>[4x]FQSMNRSALDFRHFVDHLRRQGDLVDVHTEVDANLEIGAITRRVYERRAPAPLFHNIRDSLPGARVLGAPAGLRADRARAHSRLALHFGLPEHSGPRDIVAMLRAAMRAEPIAPRRLERGPVQENVWLGEQVDLTRFPVPLLHEQDGGRYFGTYGFHVVQTPDGSWDSWSVGRLMLVDRNTLAGPTIPTQHIGIIREQWRRLGKPTPWAMALGAPPAALAAAGMPLPEGVSEAGYVGALVGEPVEVVRTQTNGLWVPANTEIVLEGEISLDETALEGPMGEYHGYSFPIGKPQPLFHVHALSFRDQPILPICVAGTPPEEHHTIWGTMISAQLLDVAQNAGLPVDMVWCSYEAATCWAVLSIDVQRLAALGTDAAAFAARVAETVFGSHAGHLVPKLILVGNDIDVTEIDQVVWALATRAHPLHDHFAFPQIRDFPMVPYLDAEDKARGSGGRLVINCLYPEQFAGQMRAATASFRHAYPTALRRRVEERWSDYGFGDA

The UbiD family of reversible (de)carboxylases depends on the recently discovered prenylated-FMN (prFMN) cofactor for activity. Here, we show that the Pseudomonas aeruginosa virulence attenuation factor PA0254/HudA is a pyrrole-2-carboxylic acid decarboxylase. We here report that the UbiD-like Pseudomonas aeruginosa virulence attenuation factor PA0254/HudA is a close homologue of Bacillus megaterium PYR2910 pyrrole-2-carboxylate (P2C) decarboxylase and show that PA0254 is capable of prFMN-dependent decarboxylation of P2C as well as carboxylation of pyrrole. Substrate screening reveals HudA and selected active site variants can accept a modest range of heteroaromatic compounds, including thiophene-2-carboxylic acid. Together with computational studies, our data suggests prFMN covalent catalysis occurs via electrophilic aromatic substitution and links HudA activity with the inhibitory effects of pyrrole-2-carboxylic acid on P. aeruginosa quorum sensing.

A number of PA0254 variants were generated in order to establish the proposed role of N318 in substrate recognition. In the case of HmfF, the corresponding residue is H297, which was established to be key to ensuring specificity for furan-type substrates. Hence, we designed a PA0235 N318H variant to test whether this would affect the substrate specificity and possibly alter the preference to furan-type substrates. Surprisingly, the purified N318H variant was found to possess an intense yellow color consistent with oxidized flavin. Structure determination of the N318H variant revealed that the introduced histidine side chain partially occupies the site of the prenyl-derived fourth prFMN ring, preventing prFMN binding. Hence, we created a series of distinct N318X variants, restricted to amino acids with a size similar to or smaller than asparagine.>[10x]DESKIAVLVVIYDHHQRELNQRMIDIQHASGTHVLCTTHIHMDEHNCLET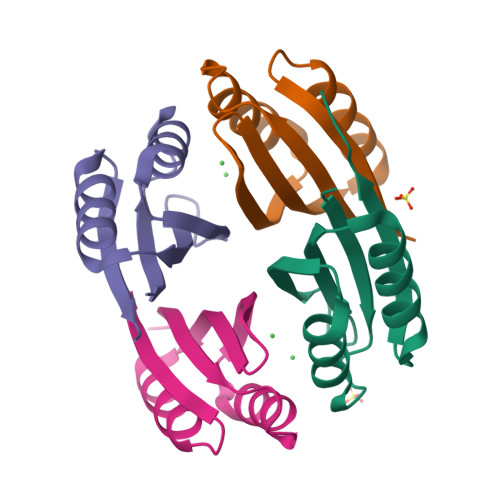IILQGNSFEIQRLQLEIGGLRGVKFAKLTKASSFEYNE>[2x]MTKITLSDLPLREELRGEHAYGAPQLNVDIRLNTNENPYPPSEALVADLVATVDKIATELNRYPERDAVELRDELAAYITKQTGVAVTRDNLWAANGSNEILQQLLQAFGGPGRTALGFQPSYSMHPILAKGTHTEFIAVSRGADFRIDMDVALEEIR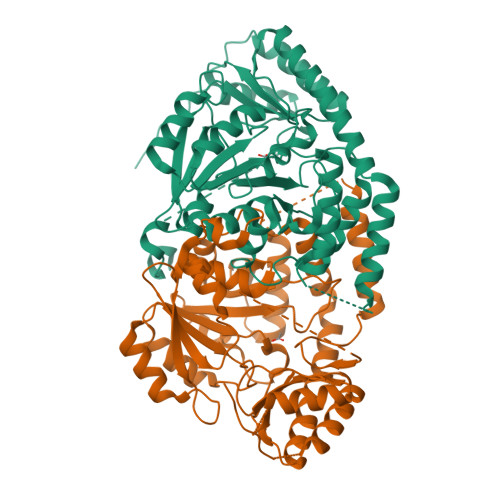AKQPDIVFVTTPNNPTGDVTSLDDVERIINVAPGIVIVDEAYAEFSPSPSATTLLEKYPTKLVVSRTMSKAFDFAGGRLGYFVANPAFIDAVMLVRLPYHLSALSQAAAIVALRHSADTLGTVEKLSVERVRVAARLEELGYAVVPSESNFVFFGDFSDQHAAWQAFLDRGVLIRDVGIAGHLRTTIGVPEENDAFLDAAAEIIKLNLSAWSHPQFEK[[(2~{R},3~{S},4~{R},5~{R})-5-(6-aminopurin-9-yl)-3,4-bis(oxidanyl)oxolan-2-yl]methoxy-oxidanyl-phosphoryl] [(3~{S},4~{R},5~{R})-3,4-bis(oxidanyl)-5-sulfanyl-oxolan-2-yl]methyl hydrogen 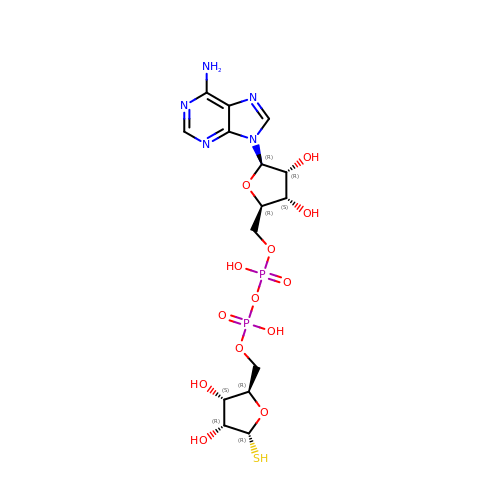phosphate | C15 H23 N5 O13 P2 S | AIFODOLMLYAQQN-KEOHHSTQSA-N> GSHMMRN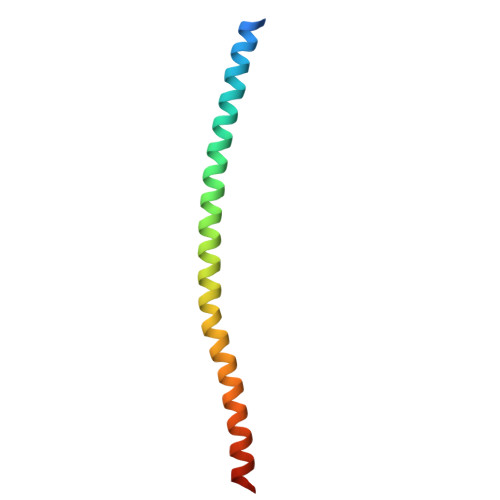ELEEMQRRADQLADESLESTRRMLQLVEESKDAGIRTLVMLDEQGEQLDRVEEGMNHINQDMKEAEKNLKDLGW>MTGAATAAENSATQLEFYRKALNFNVIGRYDPKIKQLLFHTPHASLYKWDFKKDEWNKLEYQGVLAIYLRDVSQNTNLLPVSPQEVDIFDSQNGSNNIQVNNGSDNSNRNSSGNGNSYKSNDSLTYNCGKTLSGKDIYNYGLII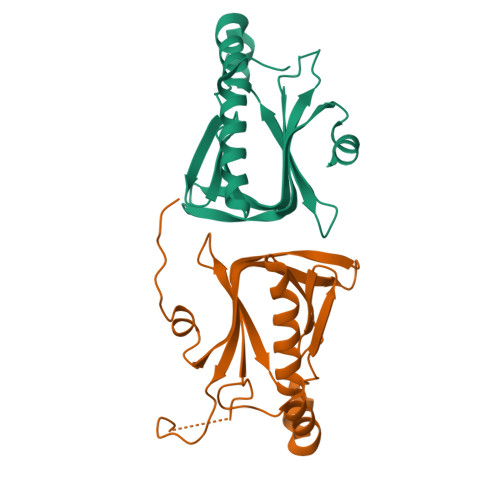LNRINPDNFSMGIVPNSVVNKRKVFNAEEDTLNPLECMGVEVKDELVIIKNLKHEVYGIWIHTVSDRQNIYELIKYLLENEPKDSFA[2x]6-methyl-1,6-dihydro-7H-pyrrolo[2,3-c]pyridin-7-one | C8 H8 N2 O 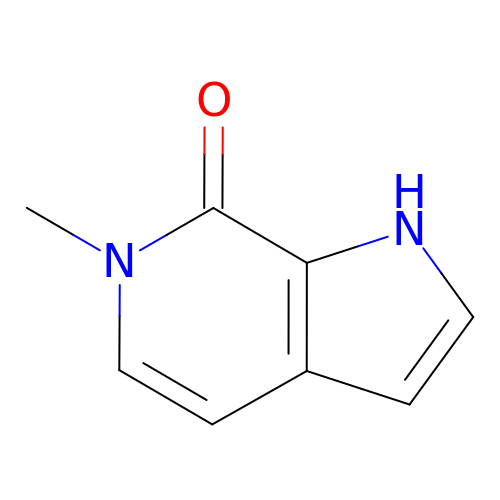| ZLKWLYKVKAVOMD-UHFFFAOYSA-N> MIKVLFFAQVRELVGTDATEVAADFPTVEALRQHMAAQSDRWALALEDGKLLAAVNQTLVSFDH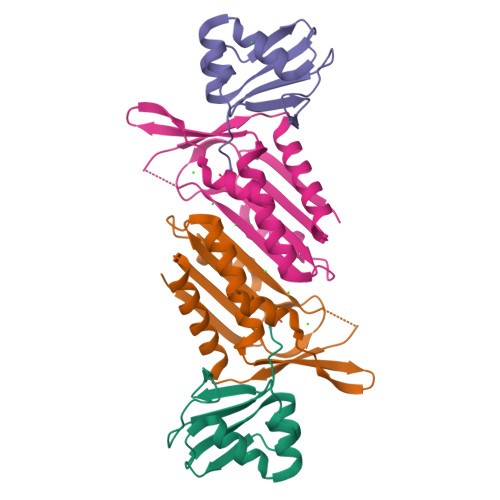PLTDGDEVAFFPPVTGG;> AETKIVVGPQPFSVGEEYPWLAERDEDGAVVTFTGKVRNHNLGDSVNALTLEHYPGMTEKALAEIVDEARNRWPLGRVTVIHRIGELWPGDEIVFVGVTSAHRSSAFEAGQFIMDYLKTRAPFWKREATPEGDRWVEARESDQQAAKRW>[2x]MSHLAELVANAAAAINQASDVAALDNVRVEYLGKKGHLTLQMTTLRDLPPEERPAAGAVINAAKEQVQQALNARKAELESAALNARLAAETIDISLPGRRIENGGLHPVTRTIDRIESFFGELGFTVATGPEIEDDYHNFDALNIPGHHPARADHDTFWFDATRLLRTQTSGVQIRTMKAQQPPIRIIAPGRVYRNDYDQTHTPMFHQMEGLIVDTNISFTNLKGTLHDFLRNFFEEDLQIRFRPSYFPFTEPSAEVDVMGKNGKWLEVLGCGMVHPNVLRNVGIDPEIYSGFAFGMGMERLTMLRYGVTDLRSFFENDLRFLKQFK;>[2x]MKFSELWLREWVNPAIDSDALANQITMAGLEVDGVEPVAGSFNGVVVGEVVECAQHPNADKLRVTKVNVGGERLLDIVCGAPNCRQGLKVAVATIGAILPGDFKIKAAKLRGEPSEGMLCSFSELGISDDHSGIIELPADAPLGTDIREYLKLDDNTIEISVTPNRADCLGIIGVARDVAVLNKAPLQEPEMAPVTATISDTLPITVEAADACPRYLGRVVKGINVNAPTPLWMKEKLRRCGIRSIDAVVDVTNYVLLELGQPMHAFDKDRIDGGIVVRMAKEGETVVLLDGSEATLNADTLVIADHHKALGIAGIFWGEHSGVNGETQNVLLECAYFNPLSIT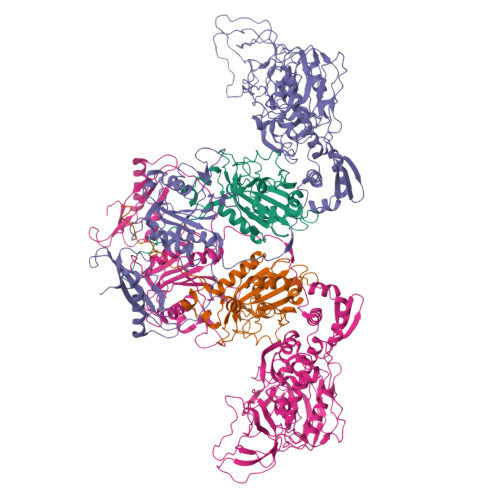GRARRHGLHTDASHRYERGVDPALQYKAIERATRLLLDICGGDAGPIIDVSNEATLPKRATITLRRSKLDRLIGHHIADEQVSDILRRLGCEVTEGQDEWKAVAPTWRFDMEIEEDLVEEVARVYGYNNIPDEPIQAGLIMGTHREADLSLKRVKTMLNDKGYQEVITYSFVDPKVQQLIHPGAEALLLPNPISVEMSAMRLSLWSGLLATVVYNQNRQQNRVRIFETGLRFVPDTQANLGIRQDLMLAGVICGNRYDEHWNLAKETVDFYDLKGDLEAVLDLTGKLGDIQFKAEMNPALHPGQSAAIYLKDERIGFIGVVHPELERKLDLNGRTLVFELEWNKLADRIVPQAREISRFPANRRDIAVVVAENVPAADILSECKKVGVNQVVGVNLFDVYRGKGVAEGYKSLAISLILQDTNRTLEEEEIAATVAKCVEALKERFQASLRD>[2x]AKLETVTLGNIGKDGKQTLVLNPRGVNPTNGVASLSQAGAVRALEKRVTVSVSQPSRNRKNYKVQVKIQNPTAGTANGSGDPSVTRQA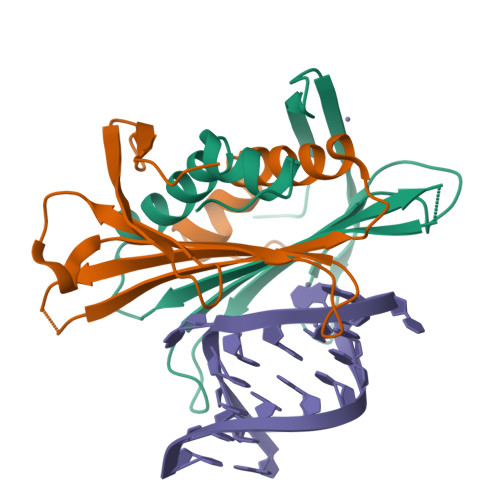YADVTFSFTQYSTDEERAFVRTELAALLASPLLIDAIDQLRPAY2-nitrophenyl beta-D-galactopyranoside | C12 H15 N O8 | 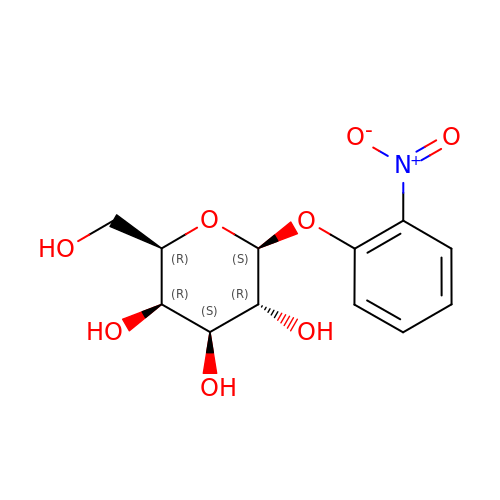KUWPCJHYPSUOFW-YBXAARCKSA-N N-[(2S)-1-[5-[2-[(4-cyanophenyl)amino]-4-(propylamino)pyrimidin-5-yl]pent-4-ynylamino]-1-oxidanylidene-propan-2-yl]-4-(dimethylamino)-N-methyl-but-2-enamide | C29 H38 N8 O2 | 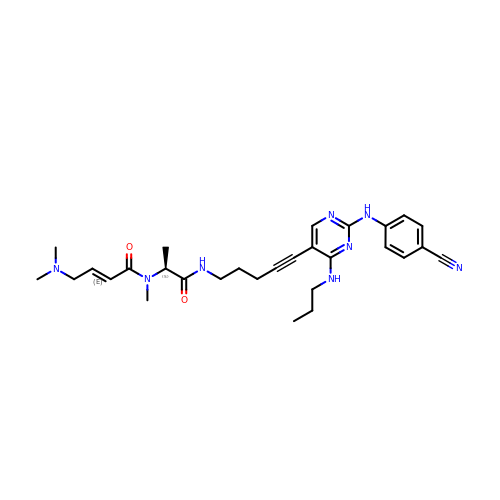HJFSVYUFOXAVAA-YUAYGMJFSA-N>SEWKARRFWASVGIHKEEGGWAVLLDERPLRTPGKQPLRLPTEALALAIAEEWQAVQEVIDPNAMPLTRSANSAIEKVAPQFDAVAAMLGDYGGTDLLSYRADAPEALVRAQAEGWDPLIDWAATELRAPLRITHGVIPVPQDPVVLLKLRAEVASLDPFGLTALHDLVTLPGSLILGLAVIRGRIDAPTAHALSRIKEEFQAERWGRDEEAEAQAASRLAAMRDSERFWHLTR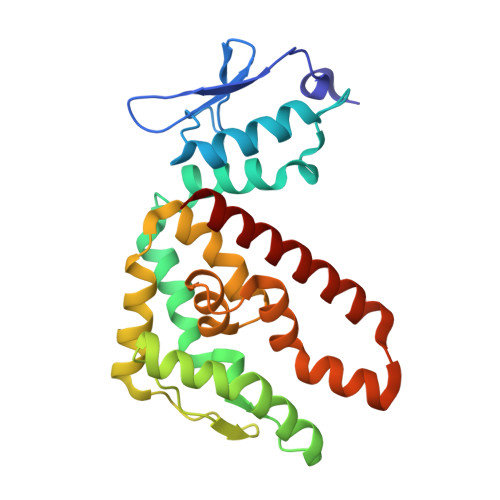[2x]>[2x]MKIVLVLYDAGKHAADEEKLYGCTENKLGIANWLKDQGHELITTSDKEGGNSVLDQHIPDADIIITTPFHPAYITKERIDKAKKLKLVVVAGVGSDHIDLDYINQTGKKISVLEVTGSNVVSAAEHVLMTMLVLVRNFVPAHEQIINHDWEVAAIAKDAYDIEGK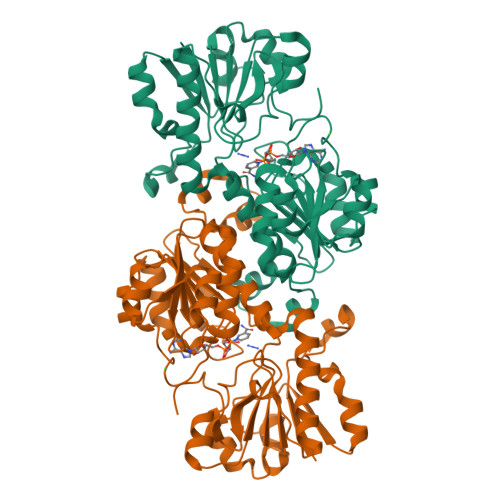TIATIGAGRIGYRVLERLVPFNPKELLYYDYQALPKDAEEKVGARRVENIEELVAQADIVTINAPLHAGTKGLINKELLSKFKKGAWLVNTARGAICVAEDVAAALESGQLRGYGGDVWFPQPAPKDHPWRDMRNKYGAGNAMTPHYSGTTLDAQTRYAEGTKNILESFFTGKFDYRPQDIILLNGEYITKAYGKHDKK>GSVGQSLQFLEMGRVTPAQFGAVGDGASHPLSERYATLAEAQTVYPHAVALSDEIDWAALQAAVDSGAPVHIPSGDYQINRGISSTGSLQIAGDGATSIIRPTAAFTGTSVLSCVGSLVALPNISSVSAGSLTIDFASTPNLVAGDVFIIYNPTDSSFSGFRTSYRAGEFCEVRAVSGNTVTIRSALYAAYDGATVAIYKVVSGVVDIASIQIVGGTVPMNGLLVEAVVSPRVDDVTVTLANNAGVYFARCYDAKITNSNISNIGDGGDDYGIIFGNCHDGGADNCKVYARRHAIATGGDAEVGCVPVRNVRMRNCTLRNDITSGTHCADFHGN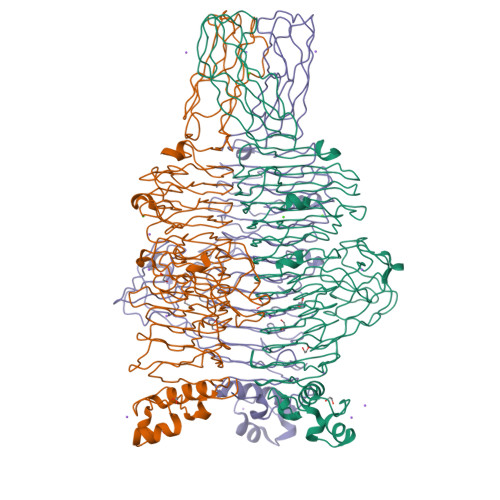AEDCSYENCTIYGGATWQGKDISYRHCTITNASGGWIVISAEILGGTFLLDQCTLYTTGDPQPGNRGVIDVGGNSAVLTTNTTQPCNFLIQGGSLRAPSLSTSSYLLRARLEGSTVPVNIQYSGQAIDVGSLGKVLQLDITSGSTSPEYLIVENLAGLPSGITLASAAGGFASAPMRMPVLGGRVQVTTATNASSVTAPVTFRYIYPKAPTVQVTKTDRSYAGNRVGVAIANPTSASGATLGLFTDDGTNFSSAVTNQLNWQAGIYEV[6x]3-({4-[(2-amino-4-oxo-4,7-dihydro-3H-pyrrolo[2,3-d]pyrimidin-5-yl)methyl]benzene-1-carbonyl}amino)-4-(carboxymethyl)benzoic 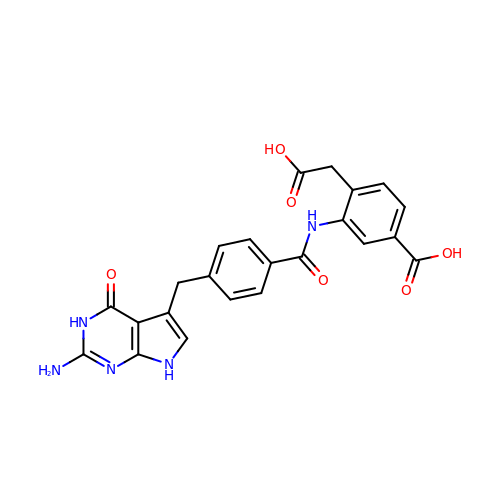acid | C23 H19 N5 O6 | FDEJWGPULAIBRF-UHFFFAOYSA-N> ENTISFFDSGDPERMNNEALMRGCGEQIVNLRPLLRTFRTINDNWSLAANTKTPITDLTNTADAEGRDYMSYLSFLYRFYRGGRRYKFFNTTPLKQSQTCYVRSFLIPRNYTADEINTDGPSHITYPVINPVHEVEVPFYSQYRKIPIASTSDKGYDSSLMYYTNVGTQQIVARAGNDDFTFGWMIGTPQLQGITKEV;> SIIQFLQRPVLIDNIEIVAGTT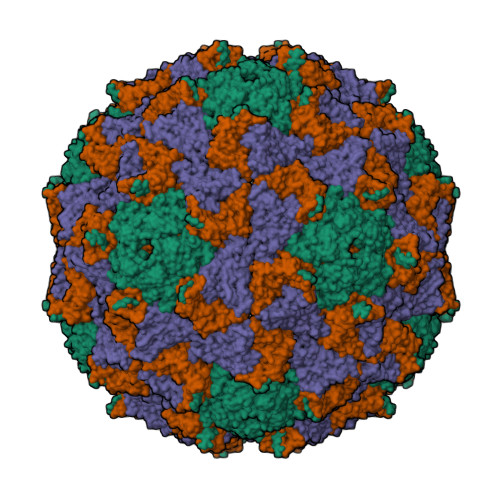ADNNTALSRYVLDRTNPQKYIKQWTLPSTVLKAGGKAQKLANFKYLRCDVQVKIVLNANPFIAGRLYLAYSPYDDKVAPERRIIYTSRAGVTGYPGVELDFQLDNSVEMTIPYASFQEAYDLVSGNEDFVQLYLFTIAPVLGPSAESANSKVDLSVYMWLDNISLVIPTYRLNP;> SKPRNQNQVMPYQNVPGWGYSLYKGIDMSVPLAYDPNNELGDLRDVFPSAVDEMAIGYVCGNPAIKHVLTWSTTDVVQNPISNGDDWGGVIPVGMPCYSKTIRAVKGATSTSKTEVMDPAPCEYVANLFSYWRATMCYRITVVKTAFHTGRLEIFFEPGSIPTVRTADNLGPDQTQLNGTIAPSDNNYKYILDLTNDTEVTIKVPYVSNKMFMKTVGIYGAHDEDNWNFDESFTGFLCIRPITKLMAPDTVSQKVSIVVWKWAEDVVVVEPKPLTSGPTQVYNPPAVA> MENTENSVDSKSIKNLEPKIIHGSESMDSGISLDNSYKMDYPEMGLCIIINNKNFHKSTGMTSRSGTDVDAANLRETFRNLKYEVRNKNDLTREEIVELMRDVSKEDHSKRSSFVCVLLSHGEEGIIFGTNGPVDLKKITNFFRGDRCRSLTGKPKLFIIQACRGTELDCGIETD;> SGVDDDMACHKIPVEADFLYAYSTAPGYYSWRNS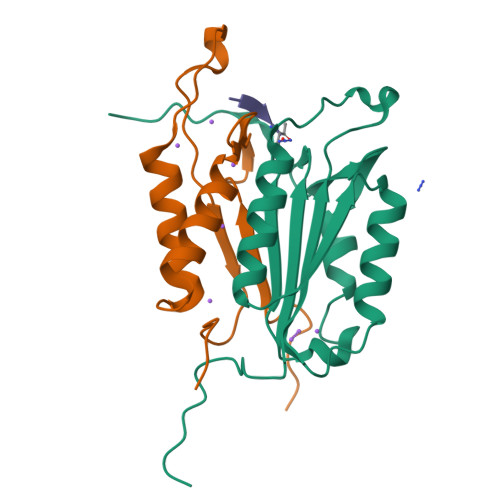KDGSWFIQSLCAMLKQYADKLEFMHILTRVNRKVADEFESFSFDATFHAKKQIPCIVSMLTKELYFYHH> SGPIDFWSSHPGQSSAAERELIGRFQDRFPTLSVKLIDAGKDYDEVAQKFNAALIGTDVPDVVLLDDRWWFHFALSGVLTALDDLFGQVGVDTTDYVDSLLADYEFNGRHYAVPYARSTPLFYYNKAAWQQAGLPDRGPQSWSEFDEWGPELQRVVGAGRSAHGWANADLISWTFQGPNWAFGGAYSDKWTLTLTEPATIAAGNFYRNSIHGKGYAAVANDIANEFATGILASAVASTGSLAGITASARFDFGAAPLPTGPDAAPACPTGGAGLAIPAKLSEERKVNALKFIAFVTNPTNTAYFSQQTGYLPVRKSAVDDASERHYLADNPRARVALDQLPHTRTQDYARVFLPGGDRIISAGLESIGLRGADVTKTFTNIQKRLQVILDRQIM;> GSGPIDFWSSHPGQSSAAERELIGRFQDRFPTLSVKLIDAGKDYDEVAQKFNAALIGTDVPDVVLLDDRWWFHFALSGVLTALDDLFGQVGVDTTDYVDSLLADYEFNGRHYAVPYARSTPLFYYNKAAWQQAGLPDRGPQSWSEFDEWGPELQRVVGAGRSAHGWANADLISWTFQGPNWAFGGAYSDKWTLTLTEPATIAAGNFYRNSIHGKGYAAVANDIANEFATGILASAVASTGSLAGITASARFDFGAAPLPTGPDAAPACPTGGAGLAIPAKLSEERKVNALKFIAFVTNPTN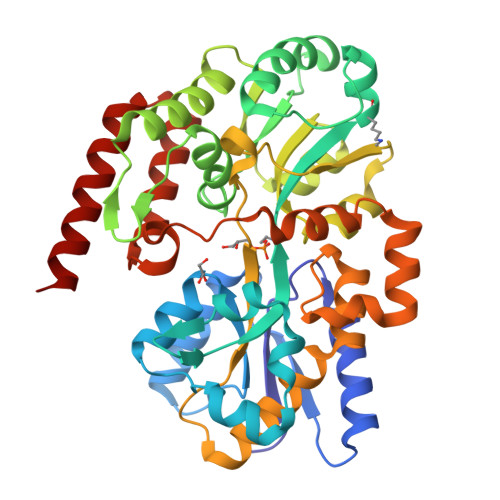TAYFSQQTGYLPVRKSAVDDASERHYLADNPRARVALDQLPHTRTQDYARVFLPGGDRIISAGLESIGLRGADVTKTFTNIQKRLQVILDRQIM;> GSGPIDFWSSHPGQSSAAERELIGRFQDRFPTLSVKLIDAGKDYDEVAQKFNAALIGTDVPDVVLLDDRWWFHFALSGVLTALDDLFGQVGVDTTDYVDSLLADYEFNGRHYAVPYARSTPLFYYNKAAWQQAGLPDRGPQSWSEFDEWGPELQRVVGAGRSAHGWANADLISWTFQGPNWAFGGAYSDKWTLTLTEPATIAAGNFYRNSIHGKGYAAVANDIANEFATGILASAVASTGSLAGITASARFDFGAAPLPTGPDAAPACPTGGAGLAIPAKLSEERKVNALKFIAFVTNPTNTAYFSQQTGYLPVRKSAVDRARVALDQLPHTRTQDYARVFLPGGDRIISAGLESIGLRGADVTKTFTNIQKRLQVILDRQIMR;> GSGPIDFWSSHPGQSSAAERELIGRFQDRFPTLSVKLIDAGKDYDEVAQKFNAALIGTDVPDVVLLDDRWWFHFALSGVLTALDDLFGQVGVDTTDYVDSLLADYEFNGRHYAVPYARSTPLFYYNKAAWQQAGLPDRGPQSWSEFDEWGPELQRVVGAGRSAHGWANADLISWTFQGPNWAFGGAYSDKWTLTLTEPATIAAGNFYRNSIHGKGYAAVANDIANEFATGILASAVASTGSLAGITASARFDFGAAPLPTGPDAAPACPTGGAGLAIPAKLSEERKVNALKFIAFVTNPTNTAYFSQQTGYLPVRKSAVDRARVALDQLPHTRTQDYARVFLPGGDRIISAGLESIGLRGADVTKTFTNIQKRLQVILDRQI The anti-apoptotic (pro-survival) proteins of the BCL-2 family include BCL-2, BCL-XL, MCL-1, BCL-w and BFL-1/A1. These proteins bind to and sequester the apoptosis effectors, as well as the apoptosis sensitizers, BIM, BID, PUMA, NOXA, BAD, BMF, HRK and BIK5,6. An elongated hydrophobic groove is thus formed along the surface of BCL-2 and BCL-XL proteins, spanning approximately 20 Å to serve as the binding site for the amphipathic α-helical BH3 domains of their pro-apoptotic partners. Herein we present cyclic peptides (CPs) with nanomolar-level binding affinities to BCL-2 or BCL-XL, and further reveal the structural and functional mechanisms of how these CPs target two proteins in a fashion that is remarkably different from traditional small-molecule inhibitors.

Because it was very difficult to obtain crystals of BCL-2 WT proteins in complex with cp2, we adopted a surface-residue mutated version of BCL-2 protein, BCL-2-12M13, which exhibits an overall three-dimensional structure as same as in the BCL-2-cp1 complex. In order to figure out how cp2 exhibits a higher binding affinity than cp1, we compared and analyzed the binding conformations of cp1 and cp2 and their surrounding key residues within 5 Å in the BCL-2 complexes. Notably, cp2 forms an additional electrostatic interaction with BCL-2 residue R110 through its E6 residue. Another clear conformational difference between cp1 and cp2 comes from the side-chain positions of cp1-E10 and cp2-F10. The BCL-2 residues around cp2-F10 are all hydrophobic ones (e.g. L201, Y202), which could be the reason why they trap the cp2-F10 in its downward position as compared with cp1-E10’s upward position. The side chains of two newly introduced residues cp2-I3 and cp2-E9 (corresponding to Y3 and A9 of cp1) are facing outwards, and thus may not participate in the cp2-protein interactions directly. Therefore, cp2-E6 seems one of the possible key factors for the enhanced affinity of cp2 as compared with cp1. We found that BCL-2 D111 residue can still form a hydrogen bond with the main-chain N atom of cp2-E6, just like with the N atom of cp1-G6.

>[2x]MDNREIVMKYISYKLSQRGYEWDAGDVEENRTEAPEGTESEVVHQTLRQAGDDFSLRYRRDFAEMSSQLHLTPGTAYASFATVVEELFRDGVNWGRIVAFFEFGGVMCVESVNREMSVLVDNIAAWMATYLNDHLHTWIQDNGGWDAFVELYG;>[2x]APIRYEWDEFC> MDDKELIEYFKSQMKEDPDMASAVAAIRTLLEFLKRDKGETIQGLRANLTSAIETLCGVDSSVAVSSGGELFLRFISLASLEYSDYSKCKKIMIERGELFLRRISLSRNKIADLCHTFIKDGATILTHAYSRVVLRVLEAAVAAKKRFSVYVTESQPDLSGKKMAKALCHLNVPVTVVLDAAVGYIMEKADLVIVGAEGVVENGGIINKIGTNQMAVCAKAQNK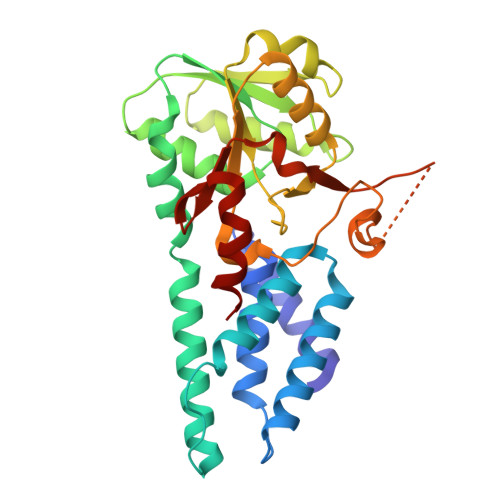PFYVVAESFKFVRLFPLNQQDVPDKFKYKADTLKVAQTGQDLKEEHPWVDYTAPSLITLLFTDLGVLTPSAVSDELIKLYL> MAAFKPNSINYILGLDIGIASVGWAMVEIDEEENPIRLIDLGVRVFERAEVPKTGDSLAMARRLARSVRRLTRRRAHRLLRTRRLLKREGVLQAANFDENGLIKSLPNTPWQLRAAALDRKLTPLEWSAVLLHLIKHRGYLSQRKNEGETADKELGALLKGVAGNAHALQTGDFRTPAELALNKFEKESGHIRNQRSDYSHTFSRKDLQAELILLFEKQKEFGNPHVSGGLKEGIETLLMTQRPALSG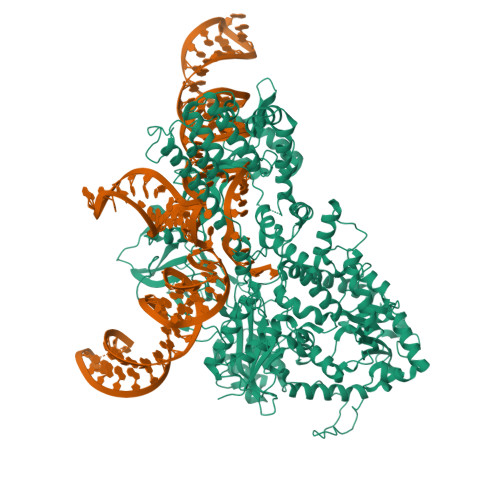DAVQKMLGHCTFEPAEPKAAKNTYTAERFIWLTKLNNLRILEQGSERPLTDTERATLMDEPYRKSKLTYAQARKLLGLEDTAFFKGLRYGKDNAEASTLMEMKAYHAISRALEKEGLKDKKSPLNLSPELQDEIGTAFSLFKTDEDITGRLKDRIQPEILEALLKHISFDKFVQISLKALRRIVPLMEQGKRYDEACAEIYGDHYGKKNTEEKIYLPPIPADEIRNPVVLRALSQARKVINGVVRRYGSPARIHIETAREVGKSFKDRKEIEKRQEENRKDREKAAAKFREYFPNFVGEPKSKDILKLRLYEQQHGKCLYSGKEINLGRLNEKGYVEIDHALPFSRTWDDSFNNKVLVLGSENQNKGNQTPYEYFNGKDNSREWQEFKARVETSRFPRSKKQRILLQKFDEDGFKERNLNDTRYVNRFLCQFVADRMRLTGKGKKRVFASNGQITNLLRGFWGLRKVRAENDRHHALDAVVVACSTVAMQQKITRFVRYKEMNAFDGKTIDKETGEVLHQKTHFPQPWEFFAQEVMIRVFGKPDGKPEFEEADTLEKLRTLLAEKLSSRPEAVHEYVTPLFVSRAPNRKMSGQGHMETVKSAKRLDEGVSVLRVPLTQLKLKDLEKMVNREREPKLYEALKARLEAHKDDPAKAFAEPFYKYDKAGNRTQQVKAVRVEQVQKTGVWVRNHNGIADNATMVRVDVFEKGDKYYLVPIYSWQVAKGILPDRAVVQGKDEEDWQLIDDSFNFKFSLHPNDLVEVITKKARMFGYFASCHRGTGNINIRIHDLDHKIGKNGILEGIGVKTALSFQKYQIDELGKEIRPCRLKKRPPVRSEHHHHHHHH>[6x]MDLLERLGLGGRRVLILHHDDLGLTHAQNGAYQALGLPTGSVMVPGAWASGVKGEDLGVHLVLTSEWPAPRMRPLTEGESLRDEAGYFPESLEALWRKARAEEVERELKAQIQAAAKLFSPTHLDAHQGAVLRPDLAEVYLRLAEAYRLVPLVPESLEGLGVPPPFLPELERLLYETPFPQVRFLDPYGLPPEERLGFYLDLAHLPPGLYYLVHHSALPTPEGRALPDW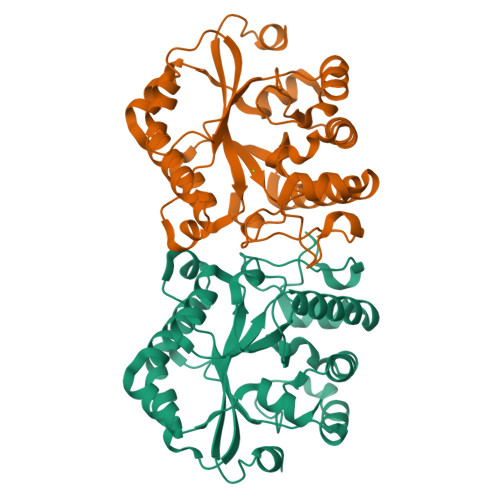PTREADYFALSHPEVRRVLAEFHPLTWRAVREALF> MRDVLTTSMARNIFYGGSLFFILIFVGLSVHSHRYIVTTSTDAATLTAEVEHGKHLWEIHGCVNCHSILGEGAYFAPELGNVMTRWGVEDDPDAAFEALKGWMDAMPTGI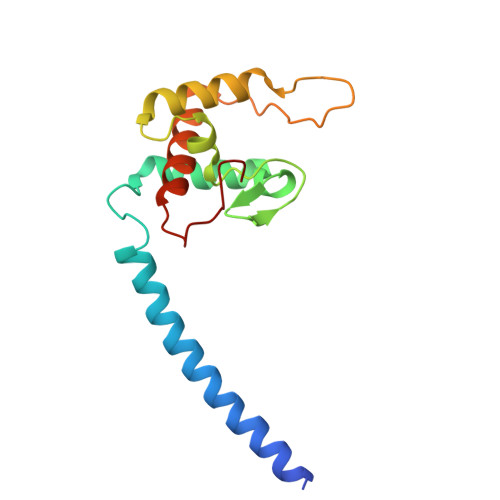EGRRQMPNFGLNDEEYRALSDFLLWTNTIRNQDWPPNDAG>MLYEEDYKLALEAFKKVFNALTHYGAKQAFRSRARDLVEEIYNSGFIPTFFYIISKAELNSDSLDSLISLFSSDNAILRGSDENVSYSAYLFIILYYLIKRGIIEQKFLIQALRCEKTRLDLIDKLYNLAPIISAKIRTYLLAIKRLSEALIEAR[3x];>MPYYAFAEPFFIHAITHLHVGSGSSVEEEIALPFQRDELGYPTIYASSLKGAIKSFLLKEFPDKRDVIYKVLGEDENPEEASLGTFLDAILFAIPSRIIEIDSAKPYVWVYVTTYELLKKVKLYLDSISQLSNASFSNLKNKIDTILAKEGKNITLDSDLKSAILNEDFYVELEALNNKIPSIINAGVPLLVLEDSIGREVINRSLIRVRRIRIDRDKKVVETGGLWSEEYVPMKTIFFSVLLGKESKESAIFASCILRNLRYVILGGKETIGKGIVELRWVKDVI[4x];> MKRVLIKPLEPLMFRSQGEFEPLITGSHTAAQSLIIPRPSTIAGMLGYILFNKSSGTGDWLSDLTNLLATIYGTFIETNGEYLFPLRMGNHLALVDQQHLINLPTLLEKEYERREKGIYELFYDKNKLFQIINHQDRIGISIDKSTRTVKEHYLYSARYLAFKKEVNYVIFIDNDAISDKINGKIVNFGGENRIAKLEVDDYKVDTSIEEEYYLALSPILIPDEALDNFLDNISDYVAMGKVDKISLGFDIANTKRKEMLTAILEGSIVKRSIIDFIKNEIKNDLRYRFSKYEKIGYNTLMSLCKLALRKILS;> MAIDFLVNILELIKEKQCNINLFSAISLTSIVYNNFGEFLSNNQSYSTNNPLLKYHIIILNDKNKTKDVEEKRNIFKREVAELISRNFKLDGEKVRNYFDSLKEVLKSLKYTIVDVEITTRTRALIGVSTSLGKLIFGSGISFDPYMNLPYIPASEIKGIVRSYIEGKLGEQEAEEIFGNEEREGNVNFTDAYPTRSKDFLFVPDVITPHYNGKKSEADAEPRPVIHLTIAPKVTFRFLIYYKREDVGKPICDSMPIILIRGLGARSSVGYSLFELRKIEVIKAAAHHHHHHHHHH;> MEELLMSLKLKALYPLTGGYNRHSINPFYEELVRPTEIKGLWRWWNRVLFNTLAYSTKGKLYTYESIDRLFEDVFGSENKKSAVRLEVITDEGNDNRFELSYVELDKVIDCLRNYKRKVSLDFIDNTLIAEIEGSTKIPISFKSNLDIDKIIKDLVHNNKLLSFELLGFKSVEIDATKISDKKILKEILRDLITNYLEYFNIKQEVTFTLNIYLDKSREHKQNFEDKLKFALYSLLVFILLGGIGRKTSRGFGSLSIIDVKCYDNSICKKIEDLAKNFLKISSGNELKSKIESILDCIKNSCIDTLYIENNILSEIDPKKNVVYFINSDLFEVKRINDKEKVLANIYKAVSSEGCCIKSIITDKYVRKSFLIAFGGYRKVEKDKGLDIGFIKNYLCETCETVSSFNIVDFLLSEGSFMSDYILQYEHRNSLLRFKLISDNSNNSYLIGYILHSSYFKKIDIKYVRCILEKLTYCVI;> MSIDNVLREFLDYKIIALLHDPPNKAWVITGRARNLTQQLSNIRASRKHEKVAKYIINQLFGKNYSEKVDNADKLASSIDRYLGSIVYKERSLFENRSIFLKNILLSNIQRDIGNLFPKDKSKLDNLILEYKKLLNVINKTNLILKYQLFYLIYELVWIDSKYENTPSDTRNPTHTIFDHLYATAAMMNWILSLEKEAKGYLLGIDTIGVADFISKGRKTRDLWISSYLVSALLWYVITWFIEEYGPDVILFPSLRFNQFYAFYLLEKLRKEGVSEDVIDEIKELITKYIFNGDDLFENLKIPPYPIIPGRITLILPGLIREGEEYKKVQDDNCFISKVKERYNEGWRKLIEGLRCYSERKREDGFWNLVCRVLKLTEDLLQTTPLNIRVKQVSVTEDEIFNNNKLRSDSWKIYDNKYRQLVSEFKKSKLVKVTPESRLKLFELTKFDKLPQIGEKSKRGYEFCTSCGVLPAVVIMPKEDELEKKLIDLGIARDEKDVRSIKNMISPGERLCPWCLVKRALGAEPRLMRILLLGDLYSVEKIVNEIVSRDVKIEIPSTSDIASIKTFEEMIEKKNEICEDLKEEEVCEKPSESVLSMWQWFNKNYYNGINLTIDPEEYWFSEKRRRYYFSVFRRHRITFPSPYYALVRADSDYLGDLLEGKLTPYLAGIIDSGDYANISEKKEEVNKLLEEYLVNAGSG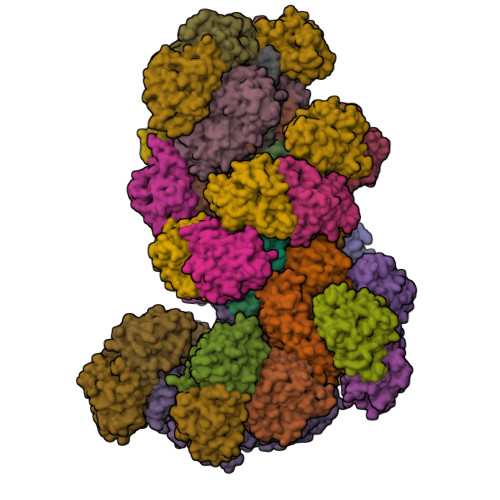SIVDYVKTVLKCIRENLNKCSCAEKIYSNEVAKVMFRVNVEKANVEEEVKNSLEYFETILNEGRIIVTPAWHVSISSALNRGLLVELELVNKHKGFVIYAGGDDLLAMLPVDEVLDFIKESRRAFAGFGTEKLGNMCLENGFVRINNAYYPSLPIVGRSYSVIIAHYADPLFFVINDSYNLLEEGKEIIRYRVMYNGEYKDAKKDVAIFRYQGLTSVIPLSLKRPIVSSVSDFNEIASIIDVILELKKRIDEGRISVSLLYDYEKYKHLIVASDEKYLTEFLVKDWIKRNSLRKHVEFTIDEKLYGVRLTIENYPIKIPNDLISNIVYTLRIIYGGEK;>MSTQREYVFIPITNSITIDVKITIGGSDHITNIDERGIHNVLVITGYAVDEKNGRLVPTLDPCDYVKGILVAGTPQQAQSNDFLTLKLPANKLYLIRKKGNISDDLKIYIPYSSPDARNSMKTKPVSISDDTIVNNIIKEVFDKIYNITQKEKVKIEKVKEDIKELFSYYALEQ[26x]> SKILVIAEHRRNDLRPVSLELIGAANGLKKSGEDKVVVAVIGSQADAFVPALSVNGVDELVVVKGSSIDFDPDVFEASVSALIAAHNPSVVLLPHSVDSLGYASSLASKTGYGFATDVYIVEYQGDELVATRGGYNQKVNVEVDFPGKSTVVLTIRPSVFKPLEGAGSPVVSNVDAPSVQSRSQNKDYVEVGGGNDIDITTVDFIMSIGRGIGEETNVEQFRELADEAGATLCCSRPIADAGWLPKSRQVGQSGKVVGSCKLYVAMGISGSIQHMAGMKHVPTIIAVNTDPGASIFTIAKYGIVADIFDIEEELK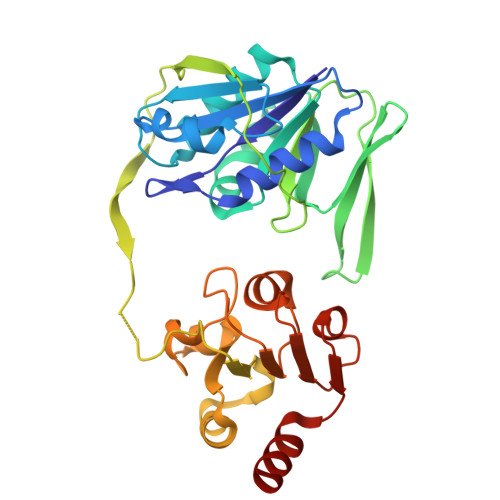AQLAA> HMLVLVAPGQGAQTPGFLTDWLALPGAADRVAAWSDAIGLDLAHFGTKADADEIRDTSVAQPLLVAAGILSAAALGTQTSVADATGPGFTPGAVAGHSVGEITAAVFAGVLDDTAALSLVRRRGLAMAEAAAVTETGMSALLGGDPEVSVAHLERLGLTPANVN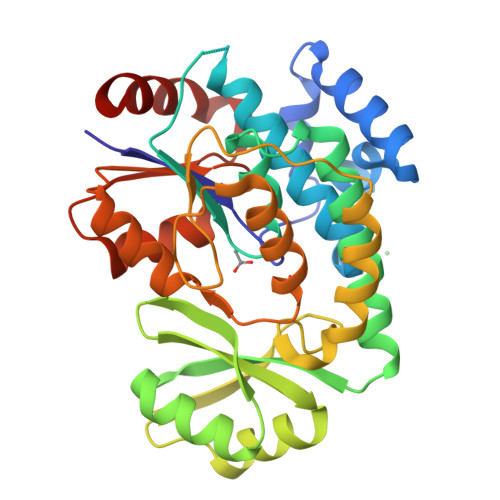GAGQIVAAGTMEQLAALNEDKPEGVRKVVPLKVAGAFHTRHMAPAVDKLAEAAKALTPADPKVTYVSNKDGRAVASGTEVLDRLVGQVANPVRWDLCMETFKELGVTAIIEVCPGGTLTGLAKRALPGVKTLALKTPDDLDAARELVAEHTQA>MAKEKGLTPQSQDFSEWYLEVIQKAELADYGPVRGTIVVRPYGYAIWENIQQVLDRMFKETGHQNAYFPLFIPMSFLRKEAEHVEGFSPELAVVTHAGGEELEEPLAVRPTSETVIGYMWSKWIRSWRDLPQLLNQWGNVVRWEMRTRPFLRTSEFLWQEGHTAHATREEAEEEVRRMLSIYARLAREYAAIPVIEGLKTEKEKFAGAVYTTTIEALMKDGKALQAGTSHYLGENFARAFDIKFQDRDLQVKYVHTTSWGLSWRFIGAIIMTHGDDRGLVLPPRLAPIQVVIVPIYKDESRERVLEAAQGLRQALLAQGLRVHLDDRDQHTPGYKFHEWELKGVPFRVELGPKDLEGGQAVLASRLGGKETLPLAALPEALPGKLDAFHEELYRRALAFREDHTRKVDTYEAFKEAVQEGFALAFHCGDKACERLIQEETTATTRCVPFEAEPEEGFCVRCGRPSAYGK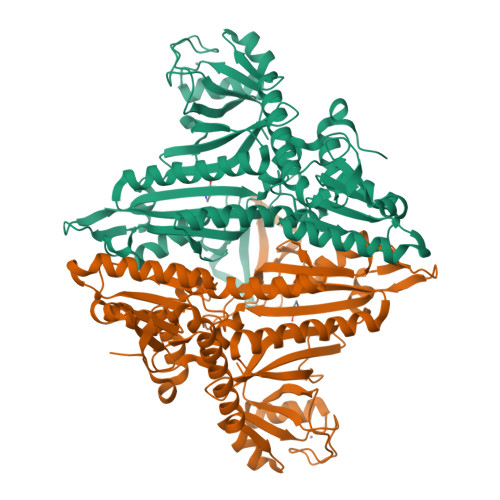RVVFAKAY[4x]> GPDSMPIDWTIEEVIQYIESNDNSLAVHGDLFRKHEID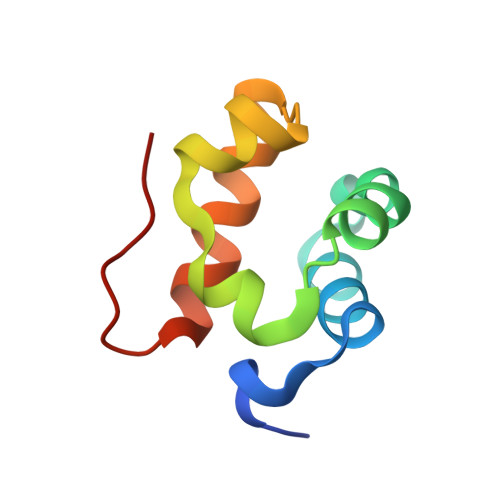GKALLLLNSEMMMKYMGLKEGPAEKICNLVNKVNGRRNNLAL> MSDSKMSSQDESKLEKAISQDSSSENHSINEYHGFDAHTSENIQNLARTFTHDSFKDDSSAGLLKYLTHMSEVPGVNPYEHEEINNDQLNPDSENFNAKFWVKNLRKLFESDPEYYKPSKLGIGYRNLRAYGVANDSDYQPTVTNALWKLATEGFRHFQKDDDSRYFDILKSMDAIMRPGELTVVLGRPGAGCSTLLKTIAVNTYGFHIGKESQITYDGLSPHDIERHYRGDVIYSAETDVHFPHLSVGDTLEFAARLRTPQNRGEGIDRETYAKHMASVYMATYGLSHTRNTNVGNDFVRGVSGGERKRVSIAEASLSGANIQCWDNATRGLDSATALEFIRALKTSAVILDTTPLIAIYQCSQDAYDLFDKVVVLYEGYQIFFGKATKAKEYFEKMGWKCPQRQTTADFLTSLTNPAEREPLPGYEDKVPRTAQEFETYWKNSPEYAELTKEIDEYFVECERSNTRETYRESHVAKQSNNTRPASPYTVSFFMQVRYGVARNFLRMKGDPSIPIFSVFGQLVMGLILSSVFYNLSQTTGSFYYRGAAMFFAVLFNAFSSLLEIMSLFEARPIVEKHKKYALYRPSADALASIISELPVKLAMSMSFNFVFYFMVNFRRNPGRFFFYWLMCIWCTFVMSHLFRSIGAVSTSISGAMTPATVLLLAMVIYTGFVIPTPSMLGWSRWINYINPVGYVFESLMVNEFHGREFQCAQYVPSGPGYENISRSNQVCTAVGSVPGNEMVSGTNYLAGAYQYYNSHKWRNLGITIGFAVFFLAIYIALTEFNKGAMQKGEIVLFLKGSLKKHKRKTAASNKGDIEAGPVAGKLDYQDEAEAVNNEKFTEKGSTGSVDFPENREIFFWRDLTYQVKIKKEDRVILDHVDGWVKPGQITALMGASGAGKTTLLNCLSERVTTGIITDGERLVNGHALDSSFQRSIGYVQQQDVHLETTTVREALQFSAYLRQSNKISKKEKDDYVDYVIDLLEMTDYADALVGVAGEGLNVEQRKRLTIGVELVAKPKLLLFLDEPTSGLDSQTAWSICKLMRKLADHGQAILCTIHQPSALIMAEFDRLLFLQKGGRTAYFGELGENCQTMINYFEKYGADPCPKEANPAEWMLQVVGAAPGSHAKQDYFEVWRNSSEYQAVREEINRMEAELSKLPRDNDPEALLKYAAPLWKQYLLVSWRTIVQDWRSPGYIYSKIFLVVSAALFNGFSFFKAKNNMQGLQNQMFSVFMFFIPFNTLVQQMLPYFVKQRDVYEVREAPSRTFSWFAFIAGQITSEIPYQVAVGTIAFFCWYYPLGLYNNATPTDSVNPRGVLMWMLVTAFYVYTATMGQLCMSFSELADNAANLATLLFTMCLNFCGVLAGPDVLPGFWIFMYRCNPFTYLVQAMLSTGLANTFVKCAEREYVSVKPPNGESCSTYLDPYIKFAGGYFETRNDGSC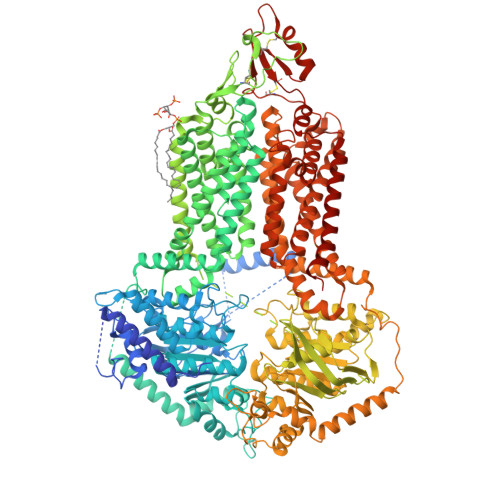AFCQMSSTNTFLKSVNSLYSERWRNFGIFIAFIAINIILTVIFYWLARVPKGNREKKNKK>TQVI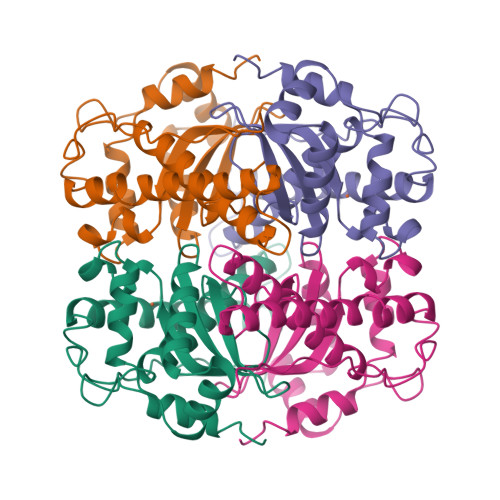QLKRYEFPQLPYKVDALEPYISKDIIDVHYNGHHKGYVNGANSLLDRLEKLIKGDLPQGQYDLQGILRGLTFNINGHKLHAIYWNNMAPAGKGGGKPGGALADLIDKQYGSFDRFKQVFSESANSLPGSGWTVLYYDNESGNLQIMTVENHFMNHIAELPVILIVDEFEHAYYLQYKNKRGDYLNAWWNVVNWDDAEKRLQKYLNK[6x]> MNRMLTLNIFRYNPLDPDSQPRMQTF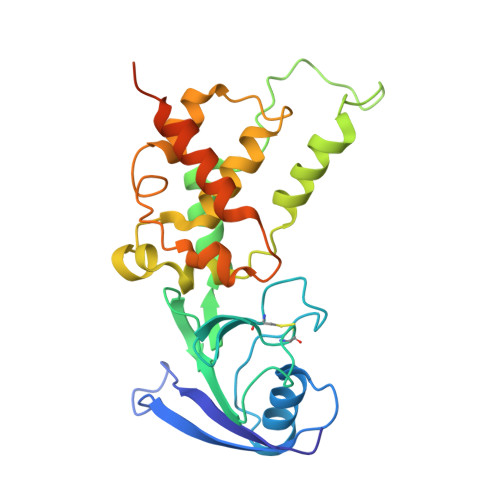TVQEYDSMTLFIALTQIRDEKDPTLKVDFCCRAGICGSCAMVINGRPGLACHTQTKDLPAEITLHPLPFFQLLGDLSVDTGSWFRKTGLQIEAWCHSDDKAFDPTADEMRMDNDLANEIFELDRCIECGCCVAACGTARMRTDFLGAVSIMRVARFYLDPRDKRSEDDYYDVIGNDQGVFGCMGLLACEDVCPKGIPLQDQLGIMRRMMAMHSVKGVLPRPLIETIKKKGCCHAHAQS> QGFSLAQYLQEQKTIVETALDQSLVITEPVTIYEAMRYSLLAGGKRLRPILCLAACEMLGGTAAMAMNTACALEMIHTMSLIHDDLPAMDNDDLRRGKPTNHKVYGEDIAILAGDALLSYAFEYVARTPDVPAERLLQVIVRLGQAVGAEGLVGGQVVDLESEGKDVAVETLNFIHTHKTGALLEVCVTAGAILAGAKPEEVQLLSRYAQNIGLAFQIVDDILDITVTYPKSQAEAQKLVAEAIASLEPYGEKANPLKALAEYIVNA;> QGFSLAQYLQEQKTIVETALDQSLVITEPVTIYEAMRYSLLAGGKRLRPILCLAACEMLGGTAAMAMNTACALEMIHTMSLIHDDLPAMDNDDLRRGKPTNHKVYGEDIAILAGDALLSYAFEYVARTPDVPAERLLQVIVRLGQAVGAEGLVGGQVVDLESETDVAVETLNFIHTHKTGALLEVCVTAGAILAGAKPEEVQLLSRYAQNIGLAFQIVDDILSLEKSQAEAQKLVAEAIASLEPYGEKANPLKALAEYI;> QGFSLAQYLQEQKTIVETALDQSLVITEPVTIYEAMRYSLLAGGKRLRPILCLAACEMLGGTAAMAMNTACALEMIHTMSLIHDDLPAMDNDDLRRGKPTNHKVYGEDIAILAGDALLSYAFEYVARTPDVPAERLLQVIVRLGQAVGAEGLVGGQVVDLESEGVETLNFIHTHKTGALLEVCVTAGAILAGAKPEEVQLLSRYAQNIGLAFQIVDDILLWGIEKSQAEAQKLVAEAIASLEPYGEKANPLKALAEYI;> QGFSLAQYLQEQKTIVETALDQSLVITEPVTIYEAMRYSLLAGGKRLRPILCLAACEMLGGTAAMAMNTACALEMIHTMSLIHDDLPAMDNDDLRRGKPTNHKVYGEDIAILAGDALLSYAFEYVARTPDVPAERLLQVIVRLGQAVGAEGLVGGQVVDLESEGKTDVAVETLNFIHTHKTGALLEVCVTAGAILAGAKPEEVQLLSRYAQNIGLAFQIVDDILTYPSLWGIEKSQAEAQKLVAEAIASLEPYGEKANPLKALAEYI;> VADAHTQGFSLAQYLQEQKTIVETALDQSLVITEPVTIYEAMRYSLLAGGKRLRPILCLAACEMLGGTAAMAMNTACALEMIHTMSLIHDDLPAMDNDDLRRGKPTNHKVYGEDIAILAGDALLSYAFEYVARTPDVPAERLLQVIVRLGQAVGAEGLVGGQVVDLESEVAVETLNFIHTHKTGALLEVCVTAGAILAGAKPEEVQLLSRYAQNIGLAFQIVKSQAEAQKLVAEAIASLEPYGEKANPLKALAEYIVNR;> QGFSLAQYLQEQKTIVETALDQSLVITEPVTIYEAMRYSLLAGGKRLRPILCLAACEMLGGTAAMAMNTACALEMIHTMSLIHDDLPAMDNDDLRRGKPTNHKVYGEDIAILAGDALLSYAFEYVARTPDVPAERLLQVIVRLGQAVGAEGLVGGQVVDLESEGKETLNFIHTHKTGALLEVCVTAGAILAGAKPEEVQLLSRYAQNIGLAFQIVDDSQAEAQKLVAEAIASLEPYGEKANPLKALAEYIVNR

In this study, we report the first crystal structure of GGPPS (CrtE) from a cyanobacterium – in our case the model strain Synechococcus sp. PCC 7002 (Syn7002). CrtE, in common with other trans-prenyltransferases, contains the two highly conserved FARM and SARM regions and contains a two amino-acid insertion (Pro-95 and Ala-96) in the FARM characteristic of a Type-II GGPPS. In the case of photosynthetic organisms, most photosynthesis-related metabolites such as carotenoids and the side chains of chlorophylls and plastoquinones are all derived from GGPP, synthesized by GGPPS. Syn7002 GGPPS is a homodimer and its three-dimensional structure is most similar to the large subunit of heterodimeric A. thaliana GGPPS1.

We obtained CrtE crystals in two different crystallization conditions. The crystal formed in 0.2 M ammonium acetate, 0.1 M sodium acetate (pH 4.6) and 30% (w/v) PEG 4000 had 6 copies in the asymmetric unit, and the crystal generated in 0.1 M sodium citrate (pH 5.5) and 20% (w/v) PEG 3000 contained 2 copies in the asymmetric unit. In both cases CrtE crystals had the same space group - P212121. Each CrtE monomer is composed of 14 α-helices (A to L, and α1) joined by connecting loops. The two aspartate-rich motifs, FARM and SARM, are located in helix D and H, respectively, forming a large catalytic cavity for allyl substrate binding. α-helices (D, E, F1, and F2) form a large tunnel-shaped pocket which is hypothesized to be involved in prenyl chain elongation according to previous structural studies. The inner surface of the pocket is filled with hydrophobic amino acids (Ala-80, Ile-84, Met-87, Leu-126, Phe-130, Leu-151, Val-155, and Leu-160) which, based on previous studies on prenyltransferase enzymes, are predicted to determine the chain length of the final product. In addition, residues in helices E, F1 and F2 at the homodimer interface are non-polar. Notably, the side chain of Phe-130 in helix E is involved in a π-π interaction with its counterpart in the other subunit, which also has been found in A. thaliana GFPPS and Sulfolobus solfataricus HexPPS. As shown in the electrostatic surface potential map, there are a number of positively charged amino acid residues (Lys-53, Arg-54, and Arg-56) located at the bottom of the catalytic cavity, which are proposed to bind the IPP substrate. Binding sites for Mg2+ and DMAPP could not be obtained in this study, but have been reported in previous structural studies of GGPPS from S. cerevisiae, Plasmodium falciparum, and Corynebacterium glutamicum.> GMQEHYQPAAIEPAAQKKWDDARISNVSEDASKPKYYCLSMFPYPSGKLHMGHVRNYTIGDVLSRFKLLNGFNVMQPMGWDAFGMPAENAAMKNNVAPAAWTYDNIEYMKTQLKSLGFAVDWEREVATCKPEYYRWEQWLFTKLFEKGIVYRKNGTVNWDPVDQTVLANGQVIDGRGWRSGALIEKREIPMYYFKITDYAEELLNDLDKLEHWPEQVKTMQRNWIGKSRGMTVRFAVSDDSKQGLEGDYAKFLQVYTTRPDTLMGATYVAVAAEHPLATAAAADKPELQAFIAECKAGSVAEADMATMEKKGVPTGRYVVNPLNGDKLEVWIANYVLWGYGDGAVMAVPAHDERDFEFAAKYNLPKKQVIAVGDNAFDANRWQEWYGDKENGVLVNSGDLDGLDFQTAFDAVAAKLQSQGAGEPKTQYRLRDWGISRQRYWGCPIPIVHCEKCGNVPVPADQLPVVLPENVVPDGMGSPLAKMPEFYETSCPCCGGAAKRETDTMDTFIESSWYFFRYMSPKFSDGMVSAESAKYWGAVDQYIGGIEHAILHLLYARFFTKLMRDEGLVNVDEPFERLLTQGMVVCETYYRENDKGGKDWINPADVELTFDDKGRPVSAVLKADGLPVVISGTEKMSKSKNNGVDPQELINAYGADTARLFMMFAAPPEQSLEWSDSGVEGAHRFLRRLWRTVYEYLKQGGAVKAFAGNQDGLSKELKDLRHKLHSTTAKVSDDYGRRQQFNTAIAAVMELLNQYDKTDTGSEQGRAVAQEVLEAAVRLLWPIVPHICETLWSELNGAKLWEAGWPTVDEAALVKSEIEVMVQVNGKLRGKITVAADASKADLEAAALANEGAVKFMEGKPAKKIIVVPGRLVNIVV

To correctly aminoacylate tRNALeu, leucyl-tRNA synthetase (LeuRS) catalyzes three reactions: activation of leucine by ATP to form leucyl-adenylate (Leu-AMP), transfer of this amino acid to tRNALeu and post-transfer editing of any mischarged product. Mechanistically similar to other adenylate-forming enzymes, the class Ia aminoacyl-tRNA synthetase (aaRS) LeuRS charges tRNALeu isoacceptors, which are essential substrates for protein translation. We have solved crystal structures for all enzymatic states of Neisseria gonorrhoeae LeuRS during Leu-AMP formation.

As the substrate-induced peptide-plane flip results from the clash with the incoming side chain of E169, we next generated a NgLeuRS-E169G mutant to investigate its corresponding effects on aminoacylation. The mutant was readily expressed and crystallized, and high-resolution structures of the NgLeuRS-E169G apo, and soaked NgLeuRS-E169G·ATP·leucinol and NgLeuRS-E169G·Leu-AMP were determined. These three structures can be fully overlaid with each other (and WT apo) with an all-atom RMSD of 0.186 Å indicating no obvious conformational changes between apo, pre-transition and intermediate states which strongly contrasts with what was observed for the WT enzyme. The interactions mediated by E169 with Y554 and W223 are thus additionally required to stabilize the closed CP1 hairpin position in the pre-transition state to promote the formation of Leu-AMP. In line with this model, independently tested amino acid activation demonstrated that substitution of E169 with a glycine results in up to fivefold increase in KM (Leu) and fourfold decrease in kcat yielding the 24-fold less efficient enzyme in Leu activation relative to the WT protein. Thus, opposite to the L550G mutant which captures the “closed conformation” and displays a defect in the aminoacyl transfer step, mutation at the CP1 hairpin which stabilizes the “open conformation” affects only the activation step.> GGRMKFTVEREHLLKPLQQVSGPLGGRPTLPILGNLLLQVADGTLSLTGTDLEMEMVARVALVQPHEPGATTVPARKFFDICRGLPEGAEIAVQLEGERMLVRSGRSRFSLSTLPAADFPNLDDWQSEVEFTLPQATMKRLIEATQFSMAHQDVRYYLNGMLFETEGEELRTVATDGHRLAVCSMPIGQSLPSHSVIVPRKGVIELMRMLDGGDNPLRVQIGSNNIRAHVGDFIFTSKLVDGRF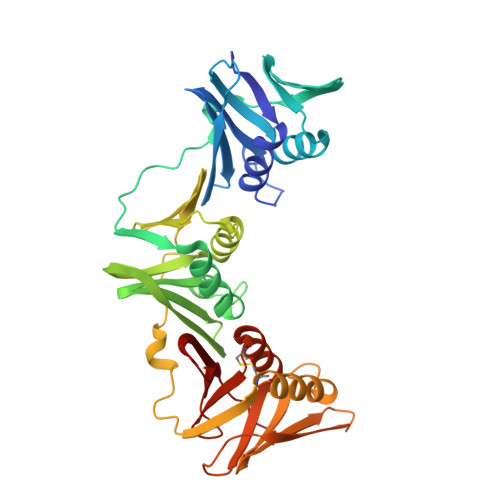PDYRRVLPKNPDKHLEAGCDLLKQAFARAAILSNEKFRGVRLYVSENQLKITANNPEQEEAEEILDVTYSGAEMEIGFNVSYVLDVLNALKCENVRMMLTDSVSSVQIEDAASQSAAYVVMPMRL> ASVKDTYTDRLDDWNGIIAGNQYYDSKNDQMAKLNQELEGKVADSLSSISSQADRIYLWEKFSNYKTSANLTATYRKLEEMAKQVTNPSSRYYQDETVVRTVRDSMEWMHKHVYNSEKSIVGNWWDYEIGTPRAINNTLSLMKEYFSDEEIKKYTDVIEKFVPDPEHFRKTTDNPFKALGGNLVDMGRVKVIAGLLRKDDQEISSTIRSIEQVFKLVDQGEGFYQDGSYIDHTNVAYTGAYGNVLIDGLSQLLPVIQKTKNPIDKDKMQTMYHWIDKSFAPLLVNGELMDMSRGRSISRANSEGHVAAVEVLRGIHRIADMSEGETKQRLQSLVKTIVQSDSYYDVFKNLKTYKDISLMQSLLSDAGVASVPRTSYLSAFNKMDKTAMYNAEKGFGFGLSLFSSRTLNYEHMNKENKRGWYTSDGMFYLYNGDLSHYSDGYWPTVNPYKMPGTTETDAKRADSDTGKVLPSAFVGTSKLDDANATATMDFTNWNQTLTAHKSWFMLKDKIAFLGSNIQNTSTDTAATTIDQRKLESSNPYKVYVNDKEASLTEQEKDYPETQSVFLESSDSKKNIGYFFFKKSSISMSKALQKGAWKDINEGQSDKEVENEFLTISQAHKQNGDSYGYMLIPNVDRATFNQMIKELESSLIENNETLQSVYDAKQGVWGIVKYDDSVSTISNQFQVLKRGVYTIRKEGDEYKIAYYNPETQES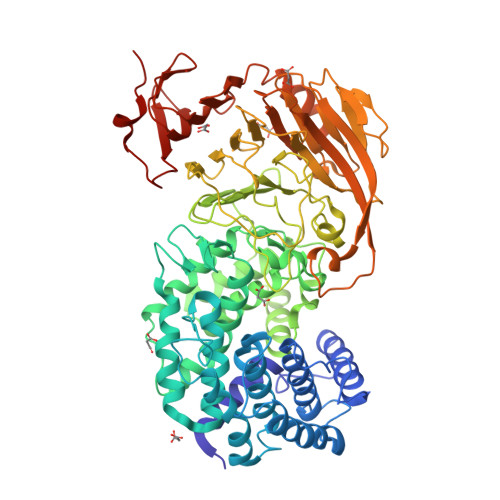APDQEVFKKLEQHHHHHH> MDGHNQNQYQNQNQIQQSQQPPLKKYVTQRRSVDVSSPYINLYYNRRHGLPNLVVEPETSYTIDIMPPNAYRGRDRVINLPSKFTHLSSNKVKHVIPAIQWTPEGRRLVVATYSGEFSLWNASSF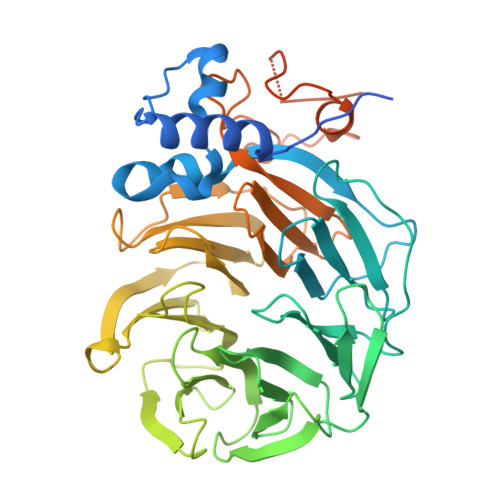TFETLMQAHDSAVTTMKYSHDSDWMISGDADGMIKIWQPNFSMVKEIDAAHTESIRDMAFSSNDSKFVTCSDDNILKIWNFSNGKQERVLSGHHWDVKSCDWHPEMGLIASASKDNLVKLWDPRSGNCISSILKFKHTVLKTRFQPTKGNLLMAISKDKSCRVFDIRYSMKELMCVRDETDYMTLEWHPINESMFTLACYDGSLKHFDLLQNLNEPILTIPYAHDKCITSLSYNPVGHIFATAAKDRTIRFWTRARPIDPNAYDDPTYNNKKINGWFFGINNDINAVREKSEFGAAPPPPATLEPHALPNMNGFINKKPRQEIPGIDSNIKSSTLPGLSI>EFSQLLALASLLGQQQAEIQR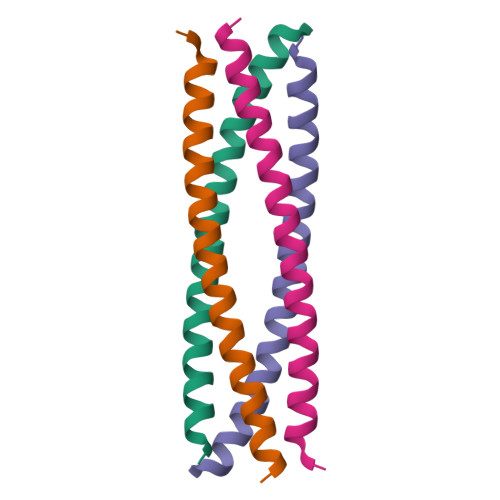CREDLQKKESLMMETIAKIKALALEHHHH[2x]N~1~-{(1S,2S,4S)-1-(cyclohexylmethyl)-4-[(2,2-dimethylpropyl)carbamoyl]-2-hydroxy-5-methylhexyl}-N~2~-(quinolin-2-ylcarbonyl)-L-aspartamide | C34 H51 N5 O5 | 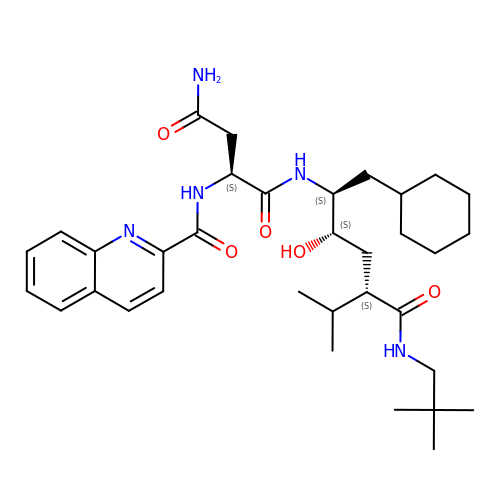YFPJVAMWHSOWMB-JSRHHAARSA-N> GPLGSVASAYAALPSWIAYEKARADLEEAKKNDVSPQLLKQLTKACNIAKSEFEREA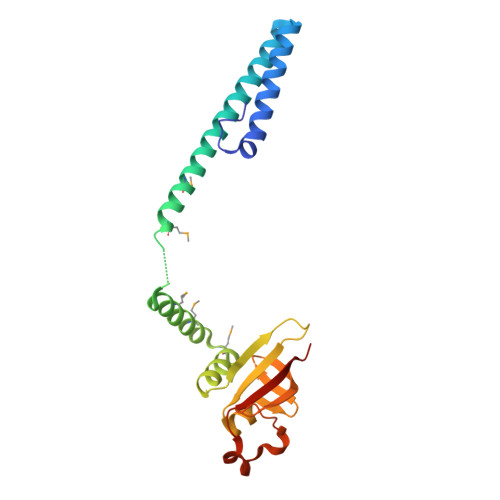SVQKKLDKMAEQAAASMYKEARAVDRKSKIVSAMHSLLFGMLKKLDMSSVNTIIEQARNGVLPLSIIPAASATRLIVVTPNLEVLSKVRQENNVHYAGAIWSIVEVKDANGAQVHLKEVTAANELNITWPLSITCERTTKLQ>[3x]GEPLYTEQDLAVNGREGFPNYRIPALTVTPDGDLLASYDGRPTGIDAPGPNSILQRRSTDGGRTWGEQQVVSAGQTTAPIKGFSDPSYLVDRETGTIFNFHVYSQRQGFAGSRPGTDPADPNVLHANVATSTDGGLTWSHRTITADITPDPGWRSRFAASGEGIQLRYGPHAGRLIQQYTIINAAGAFQAVSVYSDDHGRTWRAGEAVGVGMDENKTVELSDGRVLLNSRDSARSGYRKVAVSTDGGHSYGPVTIDRDLPDPTNNASIIRAFPDAPAGSARAKVLLFSNAASQTSRSQGTIRMSCDDGQTWPVSKVFQPGSMSFSTLTALPDGTYGLLYEPGTGIRYANFNLAWLGGICAPFTIPDVALEPGQQVTVPVAVTNQSGIAVPKPSLQLDASPDWQ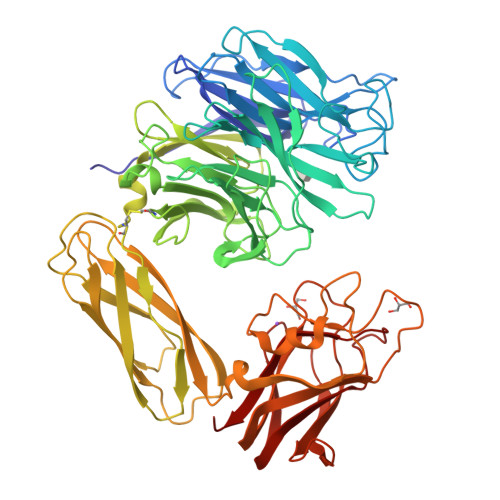VQGSVEPLMPGRQAKGQVTITVPAGTTPGRYRVGATLRTSAGNASTTFTVTVGLLDQARMSIADVDSEETAREDGRASNVIDGNPSTFWHTEWSRADAPGYPHRISLDLGGTHTISGLQYTRRQNSANEQVADYEIYTSLNGTTWDGPVASGRFTTSLAPQRAVFPARDARYIRLVALSEQTGHKYAAVAELEVEGQR> MERTVVETRYGRLRGEMNEGVFVWKGIPYAKAPVGERRFLPPEPPDAWDGVREATSFGPVVMQPSDPIFSGLLGRMSEAPSEDGLYLNIWSPAADGKKRPVLFWIHGGAFLFGSGSSPWYDGTAFAKHGDVVVVTINYRMNVFGFLHLGDSFGEAYAQAGNLGILDQVAALRWVKENIAAFGGDPDNITIFGESAGAASVGVLLSLPEASGLFRRAMLQSGSGSLLLRSPETAMAMTERILDKAGIRPGDRERLLSIPAEELLRAALSLGPGVMYGPVVDGRVLRRHPIEALRYGAASGIPILIGVTKDEYNLFTLTDPSWTKLGEKELLDRINREVGPVPEEAIRYYKETAEPSAPTWQTWLRIMTYRVFVEGMLRTADAQAAQGADVYMYRFDYETPVFGGQLKACHALELPFVFHNLHQPGVANFVGNRPEREAIANEMHYAWLSFARTGDPNGAHLPEAWPAYTNERKAAFVFSAASHVEDDPFGRERAAWQ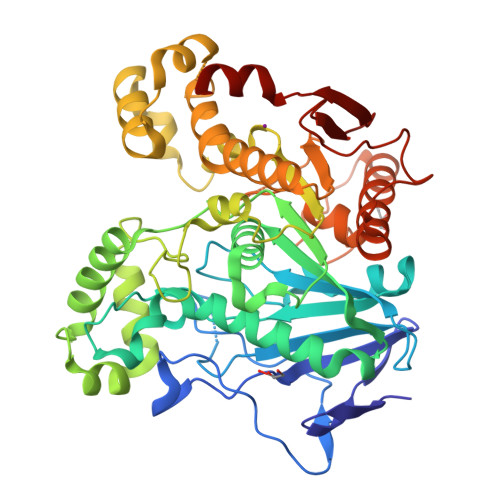GR> MSKTRVIYPGTFDPITNGHVDLVTRASRMFDEVVVAIAIGHHKNPLFSLEERVALAQSSLGHLSNVEFVGFDGLLVNFFKEQKATAVLRGLRAVSDFEYEFQLANMNRQLDPHFEAVFLTPSEQYSFISSTLIREIAR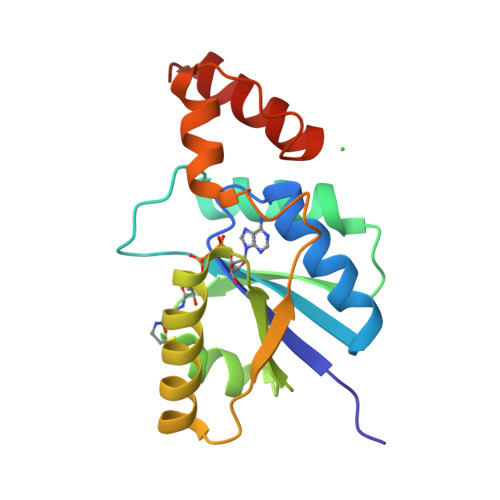LKGDVTKFVPQAVVEAFERKHQQGW>MLVFIDDGSTNIKLQWQESDGTIKQHISPNSFKREWAVSFGDKKVFNYTLNGEQYSFDPISPDAVVTTNIAWQYSDVNVVAVHHALLTSGLPVSEVDIVCTLPLTEYYDRNNQPNTENIERKKANFRKKITLNGGDTFTIKDVKVMPESIPAGYEVLQELDELDSLLIIDLGGTTLDISQVMGKLSGISKIYGDSSLGVSLVTSAVKDALSLARTKGSSYLADDIIIHRKDNNYLKQRINDENKISIVTEAMNEALR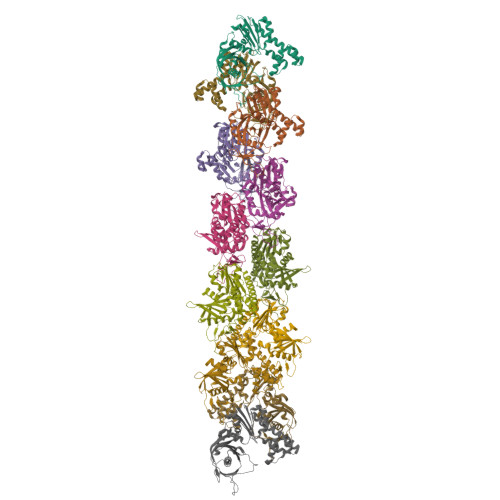KLEQRVLNTLNEFSGYTHVMVIGGGAELICDAVKKHTQIRDERFFKTNNSQYDLVNGMYLIGN[12x]>[2x]MDENAKEPENRFLRKLLKPDIERERLKAVNSIISIVFGTRRIAWAHLDRKLTVLDWQQSDRWSLMRGIYSSSVYLEEISSIISKMPKADFYVLEKTGLSIQNSSLFPILLHFHIMEAMLYALLNKTFAQDGQHQVLSMNRNAVGKHFELMIGDSRTSGKELVKQFLFDSILKADPRVFFPSDKIVHYRQMFLSTELQRVEELYDSLLQAIAFYELAVFDSQPLEHHHHHHHH;> MGHHHHHHGRWAKILEKDKRTQQMRMQRLKAKLQMPFQSGEFKALTRRLQVEPRLLSKQMAGCLEDCTRQAPESPWEEQLARLLQEAPGKLSLDVEQAPSGQHSQAQLSGQQQRLLAFFKCCLLTDQLPLAHHLLVVHHGQRQKRKLLTLDMYNAVMLGWARQGAFKELVYVLFMVKDAGLTPDLLSYAAALQCMGRQDQDAGTIERCLEQMSQEGLKLQALFTAVLLSEEDRATVLKAVHKVKPTFSLPPQLPPPVNTSKLLRDVYAKDGRVSYPKLHLPLKTLQCLFEKQLHMELASRVCVVSVEKPTLPSKEVKHARKTLKTLRDQWEKALCRALRETKNRLEREVYEGRFSL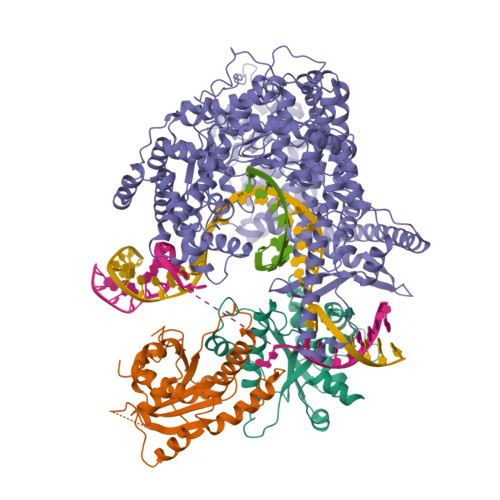YPFLCLLDEREVVRMLLQVLQALPAQGESFTTLARELSARTFSRHVVQRQRVSGQVQALQNHYRKYLCLLASDAEVPEPCLPRQYWEALGAPEALREQPWPLPVQMELGKLLAEMLVQATQMPCSLDKPHRSSRLVPVLYHVYSFRNVQQIGILKPHPAYVQLLEKAAEPTLTFEAVDVPMLCPPLPWTSPHSGAFLLSPTKLMRTVEGATQHQELLETCPPTALHGALDALTQLGNCAWRVNGRVLDLVLQLFQAKGCPQLGVPAPPSEAPQPPEAHLPHSAAPARKAELRRELAHCQKVAREMHSLRAEALYRLSLAQHLRDRVFWLPHNMDFRGRTYPCPPHFNHLGSDVARALLEFAQGRPLGPHGLDWLKIHLVNLTGLKKREPLRKRLAFAEEVMDDILDSADQPLTGRKWWMGAEEPWQTLACCMEVANAVRASDPAAYVSHLPVHQDGSCNGLQHYAALGRDSVGAASVNLEPSDVPQDVYSGVAAQVEVFRRQDAQRGMRVAQVLEGFITRKVVKQTVMTVVYGVTRYGGRLQIEKRLRELSDFPQEFVWEASHYLVRQVFKSLQEMFSGTRAIQHWLTESARLISHMGSVVEWVTPLGVPVIQPYRLDSKVKQIGGGIQSITYTHNGDISRKPNTRKQKNGFPPNFIHSLDSSHMMLTALHCYRKGLTFVSVHDCYWTHAADVSVMNQVCREQFVRLHSEPILQDLSRFLVKRFCSEPQKILEASQLKETLQAVPKPGAFDLEQVKRSTYFFS>[2x]MPVTLEPMPPGEGAQEGEPPTVEARYKSFSIKMLK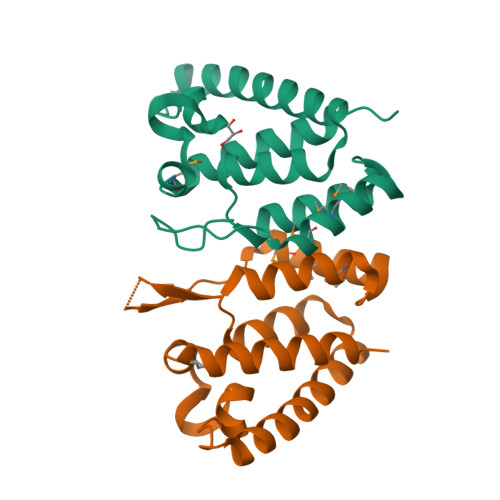DMKEGVKQYGPNSPYMRTLLDSIAHGHRLIPYDWEILAKSSLSPSQFLQFKTWWIDGVQEQVRRNRAANPPVNIDADQLLGIGQNWSTISQQALMQNEAIEQVRAICLRAWEKIQDPLEHHHHHH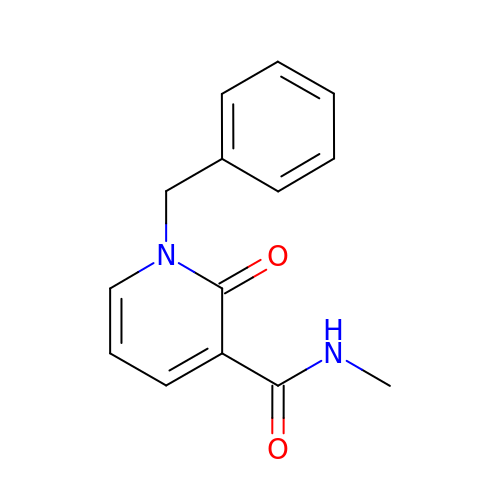~{N}-methyl-2-oxidanylidene-1-(phenylmethyl)pyridine-3-carboxamide | C14 H14 N2 O2 | FPNFBPWMDHIOEK-UHFFFAOYSA-N Rhodopseudomonas palustris propanediol utilization protein (RpPduP) reduces propionyl-CoA to propionaldehyde and shows promiscuous activity with acetyl-CoA and other CoA-ester substrates. Nevertheless, the observed promiscuous activity suggested that RpPduP could be engineered into an NADPH-dependent glycolyl-CoA reductase (GCR). Thus, to realize a carbon-neutral photorespiration bypass, the reductase should be engineered to preferentially use NADPH over NADH so that reduction is favored over oxidation.

The variant with the highest specificity toward NADPH had four mutations: P222G, I257R, N261L, and I280L. We then carried out a second round of saturation mutagenesis at second-shell sites (T196, N197, A296, L481) and identified a variant with four mutations in the acyl binding pocket (L326I, P327T, V329T, and L481H) in addition to the four mutations in the NADPH site. This variant, named GCR exhibited NADPH preference as well as ∼12-fold improved selectivity for glycolyl-CoA over acetyl-CoA compared with wild-type RpPduP (in terms of kcat/KM ratios with NADPH). The X-ray crystal structure of GCR shows that binding to NADPH is facilitated by interaction of R257 with the 2′-phosphate of NADPH and that binding to glycolyl-CoA is mediated by three mutations to polar amino acids (T327, T329, and H481), which may form two new hydrogen bonds with the hydroxyl group of the glycolyl moiety. In GCR, R257 (Ile in wild-type RpPduP) facilitates NADP(H) binding by a π-stacking interaction with the adenine ring and also, a charge–charge interaction with the 2′-phosphate group. However, the GCR crystal structure also revealed alternative binding modes where the adenosine-2′-phosphate moiety assumes different positions. Nevertheless, in these cases, the nicotinamide moiety is still correctly positioned to catalyze the reduction reaction, and this structural heterogeneity may contribute to GCR’s cofactor promiscuity. Our final engineered variant, GCR, exhibited a 1.1-fold preference for NADPH over NADH. Although the evolved enzyme accepts both NADH and NADPH, the obtained shift in specificity was sufficient to prevent the reversal of the reaction even in the presence of equimolar NAD+. The kcat of GCR with glycolyl-CoA and NADPH is similar to that of Rubisco (∼3 s−1), and its affinity toward these substrates is not limiting (KM < 0.5 mM).

>MAHHHHHHVGTNDANIADVVTKVLGEYGAPGAVSVAALTAKSPDGKSNSSADADVVARMVAKAIRDHAGTAQPSGNAATSSAAVSDGVFETMDAAVEAAALAQQQYLLCSMSDRARFVQGIRDVILNQDTLEKMSRMAVEETGMGNYEHKLIKNRLAGEKTPGIEDLTTDAFSGDNGLTLVEYSPFGVIGAITPTTNPTETIVCNSIGMLAAGNSVVFSPHGRARQVSLLLVRLINQKLAALGAPENLVVTVEKPSRENTLAMMAHPKVRMLVATGGPALVKAVLSTGKKAIGAGAGNPPVVVDETANIEKAACDIVNGCSFDNNITCTAEKEIIAVAQIADYLIFNLKKNGAYEIKDPAVLQQLQDLVLTAKGGPQTKCVGKSAVWLLSQIGISVDASIKIILMEVPREHPFVQEELMMPILPLVRVETVDDAIDLAIEVEHDNRHTAIMHSTDVRKLTKMAKLIQTTIFVKNGPSYAGHGAGGEGYSTFTIAGPTGEGLTSAKSFARRRKCVMVEALNIR[10x]> MGFITGAFFDILEVGPKKIRRCFELVRVRFAPSPTGHLHVGGARTALFNWMFARKEGGKFILRIEDTDTERSSREYEQQILESLRWCGLDWDEGPDIGGDFGPYRQSERLEIYREYAEKLVEDKRAYYVVYDKEDPSKELFTTYEYPHEYKEKGHPVTIKFKVLPGKTSFEDLLKGYMEFDNSTLEDFIIMKSNGFPTYNFAVVVDDHLMRISHVFRGEDHLSNTPKQLMIYEAFGWEAPVFMHIPLILGSDRTPLSKRHGATSVEHFRREGILSRALMNYLALLGWRVEGDEIFTIEEKLQSFDPKDISNKGVIFDYQKLEWVNGKHMRRIDLEDLKREFIEWAKYAGKEIPSVDERYFSETLRICREKVNTLSQLYDIMYPFMNDDYEYEKDYVEKFLKREEAERVLEEAKKAFKDLNSWNMEEIEKTLRDLSEKGLASKKVVFQLIRGA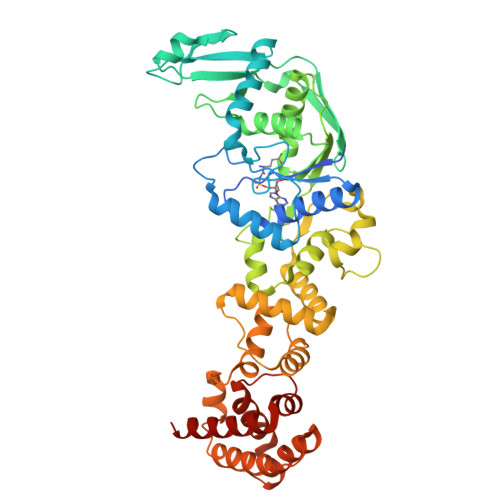VTGKLVTPGLFETIEVLGKERTLKRLERTLQFLKKT(1S,6R)-3-[2-(3,4-dimethoxyphenoxy)ethyl]-10-[(2-oxo-2,3-dihydro-1,3-benzothiazol-6-yl)sulfonyl]-3,10-diazabicyclo[4.3.1]decan-2-one | C25 H29 N3 O7 S2 | 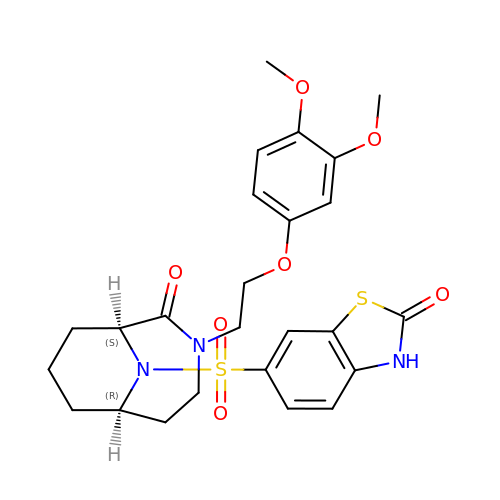ZRLORMGNOHTVCB-UZLBHIALSA-N>SEFMKIAIAGAGAMGSRFGVKLQEAGNQVTLIDNW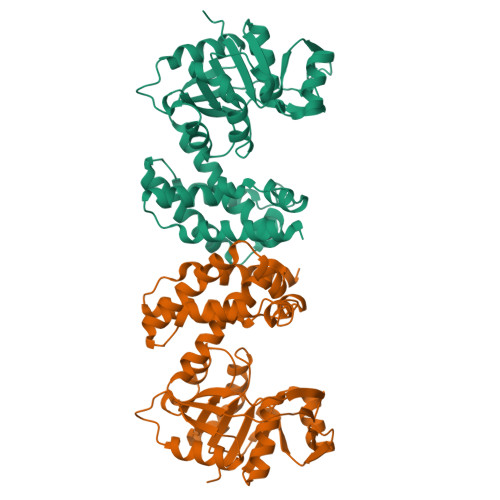SAHVDQINQAGLTVTTDDGVDHVYTMTAQHPEAVTDQFDLIILFTKTMQMDAMLQQLAPVLTNHPIVLTLANGIGNIETIERHVPKNQIVVGTTVWSSGLTGPGHITVTGTGSISLQAVVPDQFPNLADLITTLNAAGLNASAADNVLAAIWKKAGLNSVLNTYCTLFDCNIGEFGALKNWQTLTATVLDEFQAVADAAQIQFSAAAVTDWIAAQFPAAVNGNHYPSMHQDMANQRPTEIDFLNGYVAKLGQQLHVPTPANALLTQLIHSQEQLKQI[2x]N-{[(4-cyanophenyl)methyl]sulfonyl}-1-(thiophen-3-yl)cyclohexane-1-carboxamide | C19 H20 N2 O3 S2 | 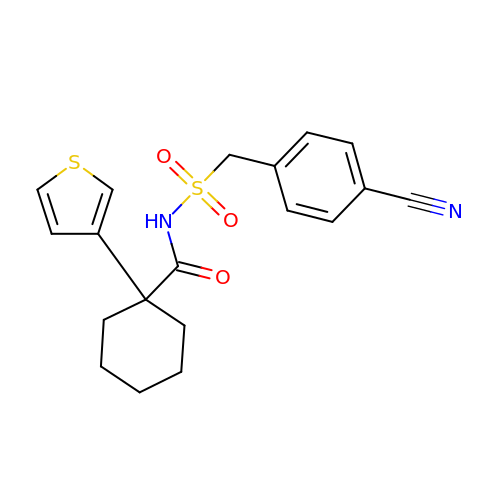KAEXAGMLFGNNER-UHFFFAOYSA-N>GLVPRGSHMTGLFVTLEGPEGAGKSTNRDYLAERLRERGIEVQLTREPGGTPLAERIRELLLAPSDEPMAADTELLLMFAARAQHLAGVIRPALARGAVVLCDRFTDATYAYQGGGRGLPEARIAALESFVQ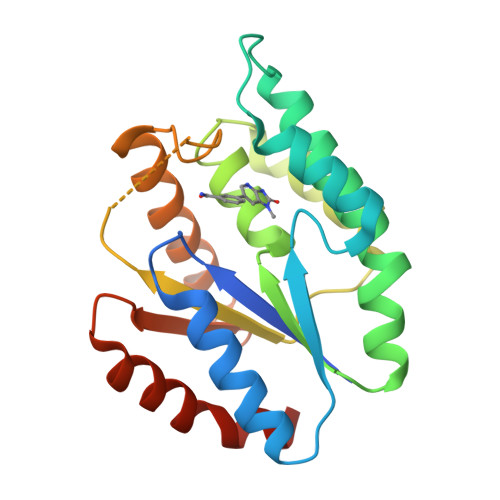GDLRPDLTLVFDLPVEIGLARAAARGRLDRFEQEDRRFFEAVRQTYLQRAAQAPERYQVLDAGLPLAEVQAGLDRLLPNLLERLNGGS[2x]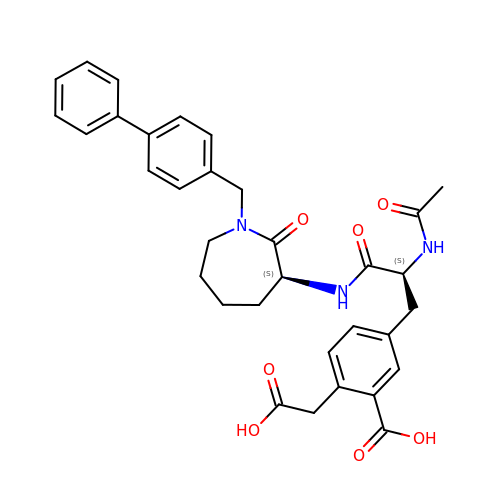5-[2-ACETYLAMINO-2-(1-BIPHENYL-4-YLMETHYL-2-OXO-AZEPAN-3-YLCARBAMOYL)-ETHYL]-2-CARBOXYMETHYL-BENZOIC ACID | C33 H35 N3 O7 | CEKLBQMULVLLTD-VMPREFPWSA-N N-{4-[(3,5-difluorophenyl)sulfonyl]benzyl}imidazo[1,2-a]pyridine-6-carboxamide | C21 H15 F2 N3 O3 S | 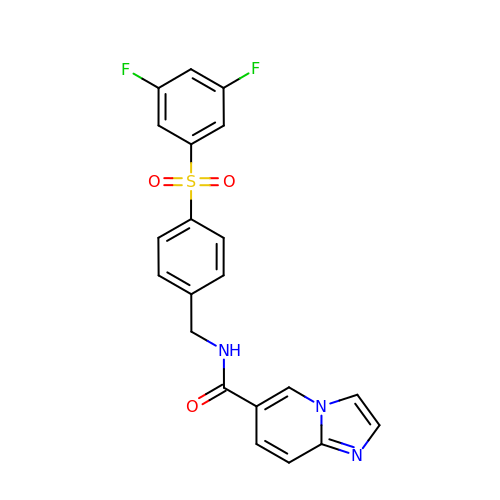XRDVXQQZLHVEQZ-UHFFFAOYSA-N> DTAWERYKARFMMPDGRIIDTANGNVSHTEGQGFAMLLAVANNDRPAFDKLWQWTDSTLRDKSNGLFYWRYNPVAPDPIADKNNASDGDTLIAWALLRAQKQWQDKRYAIASDAITASLLKYTVVTFAGRQVMLPGVKGFNLNDHLNLNPSYFIFPAWRAFAERTHLTAWRTLQTDGQALLGQMGWGKSHLPSDWVALRADGKMLPAKEWPPRMSFDAIRIPLYLSWADPQSALLAPWKAWMQSYPRLQTPAWINVSTNEVAPWYMAGGLLAVRDLTLGEPQEAPQIDDKDDYYSASLKQLVWLAKQDQR

Here, we present the cloning, expression, purification, crystallization and X-ray diffraction analysis of a cellulase from the cellulolytic bacterium K. pneumoniae found in the gut of the Chinese bamboo rat. A cellulase gene was cloned from the Klebsiella 10 chromosomal DNA using a pair of special primers and was thus named Cel10. The gene encodes a protein of 310 amino-acid residues, including a signal-peptide segment (residues 1–23), and has a mature molecular weight of 35 kDa. However, Cel10 cellulase activity was more efficient on CMC than on Avicel and xylan, which indicates that it is an endoglucanese.

There is one molecule in the asymmetric unit and the final structure contains residues 24–333. However, the functional role of this stable protrusion, which differs from that in the corresponding part of CtCelA, awaits further investigation. However, structural comparisons of the active sites of Cel10 and CtCelA reveal notable differences. Two of the five aromatic residues involved in stacking interactions that are critical for substrate recognition by CtCelA, corresponding to Trp205 and Tyr369 of CtCelA, are not conserved in Cel10. Phe163 of Cel10 seems to play an identical role to Trp205 of CtCelA, while a residue corresponding to Tyr369 of CtCelA is missing in the Cel10 structure, leading to a significant broadening of the cleft at the cellooligosaccharide reducing end. Consistent with the homology model of CMCax, Populus tremula × tremuloides KOR and the expected structure of AgCelC, the absence of subsite −3 of Cel10 is a common feature among cellulose biosynthesis-related endoglucanases. The absence of subsite −3 may account for the recognition of such lipid-linked oligosaccharides.Bacteria use sigma (σ) factors to recruit RNA polymerase (RNAP) to promoter regions of genes that need to be transcribed, with 60% bacteria containing at least one specialized σ factor, σ54, responsible for transcribing many stress response genes. The σ54-mediated transcription initiation requires specific AAA+ proteins (ATPases Associated with diverse cellular Activities) known as bacterial enhancer-binding proteins (bEBPs). DNA looping enables bEBP hexamers to engage and actively remodel the RNAP-σ54-DNA closed complex to convert it into an open complex. In this work we capture intermediate states of bEBPs in facilitating DNA opening and partial unfolding of σ54, and therefore link the ATPase activity to DNA opening and σ54 remodeling, which eventually lead to transcription activation.

To understand the structural basis and how DNA is stabilized in these complexes, we determined the structures of PspF1-275-RNAP-σ54-DNA containing mismatches between −11 and −8 [RPi(−11/−8)] and between −10 and −1 [RPi(−10/−1)]. In the RPi(−10/−1) complex, we also observe a range of PspF1-275 hexamer ring conformations with one resolved to higher resolution. Interestingly, in this conformation, the hexamer ring has similar tilt as that of RPi (−11/−8) at ~50° while the DNA is bent even further (>70°) compared to that RPi(−11/−8). Despite the conformational differences, similarly to RPi(−12/−11) structure, the protomer that engages with DNA is also at the highest position within the hexamer ring. In these complexes, we observe a previously unreported interaction between PspF and σ54 RpoN domain. This interaction is only possible with the tilted ring conformation, suggesting this interaction contributes to the stabilization of this ring conformation in both RPi(−11/−8) and RPi(−10/−1), giving rise to the higher-resolution reconstruction of these conformations. Given the PspF1-275 rings are in similar positions between RPi(−11/−8) and RPi(−10/−1) complexes, we could compare the relative positions of each protomer between RPi(−11/−8) and RPi(−10/−1). Compared to RPi(−11/−8), the position of the power stroke protomer (protomer 1) has shifted within the ring, with the protomer in position 2 now becoming the power stroke protomer (protomer 1 position) in, suggesting that these two complexes could represent two states as described in Fig. 3 after the hydrolysis of protomer 1. Interestingly, protomer 1 in RPi(−10/−1) is shifted significantly toward protomer 6 compared to that of RPi(−11/−8), with the distance between L1 of these two protomers reduced from 27 Å to 4 Å, consistent with our proposed mechanistic model that hydrolysis of protomer 1 at the top of the spiral causes it to relocate downward in the hexamer spiral. Significantly, we observe the σ54 N terminus is further shifted along the PspF hexamer in RPi(−11/−8) and RPi(−10/−1) compared to that of RPi(−12/−11).

>[6x]MAEYKDNLLGEANSFLEVLEQVSHLAPLDKPVLIIGERGTGKELIASRLHYLSSRWQGPFISLNCAALNENLLDSELFGHEAGAFTGAQKRHPGRFERADGGTLFLDELATAPMMVQEKLLRVIEYGELERVGGSQPLQVNVRLVCATNADLPAMVNEGTFRADLLDRLAFDVVQLPPLRERESDIMLMAEYFAIQMCREIKLPLFPGFTERARETLLNYRWPGNIRELKNVVERSVYRHGTSDYPLDDIIIDPFKRRPPEDAIAVSETTSLPTL;>MQGSVTEFLKPRLVDIEQVSSTHAKVTLEPLERGFGHTLGNALRRILLSSMPGCAVTEVEIDGVLHEYSTKEGVQEDILEILLNLKGLAVRVQGKDEVILTLNKSGIGPVTAADITHDGDVEIVKPQHVICHLTDENASISMRIKVQRGRGYVPASTRIHSEEDERPIGRLLVDACYSPVERIAYNVEAARVEQRTDLDKLVIEMETNGTIDPEEAIRRAATILAEQLEAFVDLRDVRQPEVKEEKPEFDPILLRPVDDLELTVRSANCLKAEAIHYIGDLVQRTEVELLKTPNLGKKSLTEIKDVLASRGLSLGMRLENWPPASIADE[2x];> MVYSYTEKKRIRKDFGKRPQVLDVPYLLSIQLDSFQKFIEQDPEGQYGLEAAFRSVFPIQSYSGNSELQYVSYRLGEPVFDVQECQIRGVTYSAPLRVKLRLVIYEREAPEGTVKDIKEQEVYMGEIPLMTDNGTFVINGTERVIVSQLHRSPGVFFDSDKGKTHSSGKVLYNARIIPYRGSWLDFEFDPKDNLFVRIDRRRKLPATIILRALNYTTEQILDLFFEKVIFEIRDNKLQMELVPERLRGETASFDIEANGKVYVEKGRRITARHIRQLEKDDVKLIEVPVEYIAGKVVAKDYIDESTGELICAANMELSLDLLAKLSQSGHKRIETLFTNDLDHGPYISETLRVDPTNDRLSALVEIYRMMRPGEPPTREAAESLFENLFFSEDRYDLSAVGRMKFNRSLLREEIEGSGILSKDDIIDVMKKLIDIRNGKGEVDDIDHLGNRRIRSVGEMAENQFRVGLVRVERAVKERLSLGDLDTLMPQDMINAKPISAAVKEFFGSSQLSQFMDQNNPLSEITHKRRISALGPGGLTRERAGFEVRDVHPTHYGRVCPIETPEGPNIGLINSLSVYAQTNEYGFLETPYRKVTDGVVTDEIHYLSAIEEGNYVIAQANSNLDEEGHFVEDLVTCRSKGESSLFSRDQVDYMDVSTQQVVSVGASLIPFLEHDDANRALMGANMQRQAVPTLRADKPLVGTGMERAVAVDSGVTAVAKRGGVVQYVDASRIVIKVNEDEMYPGEAGIDIYNLTKYTRSNQNTCINQMPCVSLGEPVERGDVLADGPSTDLGELALGQNMRVAFMPWNGYNFEDSILVSERVVQEDRFTTIHIQELACVSRDTKLGPEEITADIPNVGEAALSKLDESGIVYIGAEVTGGDILVGKVTPKGETQLTPEEKLLRAIFGEKASDVKDSSLRVPNGVSGTVIDVQVFTRDGVEKDKRALEIEEMQLKQAKKDLSEELQILEAGLFSRIRAVLVAGGVEAEKLDKLPRDRWLELGLTDEEKQNQLEQLAEQYDELKHEFEKKLEAKRRKITQGDDLAPGVLKIVKVYLAVKRRIQPGDKMAGRHGNKGVISKINPIEDMPYDENGTPVDIVLNPLGVPSRMNIGQILETHLGMAAKGIGDKINAMLKQQQEVAKLREFIQRAYDLGADVRQKVDLSTFSDEEVMRLAENLRKGMPIATPVFDGAKEAEIKELLKLGDLPTSGQIRLYDGRTGEQFERPVTVGYMYMLKLNHLVDDKMHARSTGSYSLVTQQPLGGKAQFGGQRFGEMEVWALEAYGAAYTLQEMLTVKSDDVNGRTKMYKNIVDGNHQMEPGMPESFNVLLKEIRSLGINIELEDE;> MKDLLKFLKAQTKTEEFDAIKIALASPDMIRSWSFGEVKKPETINYRTFKPERDGLFCARIFGPVKDYECLCGKYKRLKHRGVICEKCGVEVTQTKVRRERMGHIELASPTAHIWFLKSLPSRIGLLLDMPLRDIERVLYFESYVVIEGGMTNLERQQILTEEQYLDALEEFGDEFDAKMGAEAIQALLKSMDLEQECEQLREELNETNSETKRKKLTKRIKLLEAFVQSGNKPEWMILTVLPVLPPDLRPLVPLDGGRFATSDLNDLYRRVINRNNRLKRLLDLAAPDIIVRNEKRMLQEAVDALLDNGRRGRAITGSNKRPLKSLADMIKGKQGRFRQNLLGKRVDYSGRSVITVGPYLRLHQCGLPKKMALELFKPFIYGKLELRGLATTIKAAKKMVEREEAVVWDILDEVIREHPVLLNRAPTLHRLGIQAFEPVLIEGKAIQLHPLVCAAYNADFDGDQMAVHVPLTLEAQLEARALMMSTNNILSPANGEPIIVPSQDVVLGLYYMTRDCVNAKGEGMVLTGPKEAERLYRSGLASLHARVKVRITEYEKDANGELVAKTSLKDTTVGRAILWMIVPKGLPYSIVNQALGKKAISKMLNTCYRILGLKPTVIFADQIMYTGFAYAARSGASVGIDDMVIPEKKHEIISEAEAEVAEIQEQFQSGLVTAGERYNKVIDIWAAANDRVSKAMMDNLQTETVINRDGQEEKQVSFNSIYMMADSGARGSAAQIRQLAGMRGLMAKPDGSIIETPITANFREGLNVLQYFISTHGARKGLADTALKTANSGYLTRRLVDVAQDLVVTEDDCGTHEGIMMTPVIEGGDVKEPLRDRVLGRVTAEDVLKPGTADILVPRNTLLHEQWCDLLEENSVDAVKVRSVVSCDTDFGVCAHCYGRDLARGHIINKGEAIGVIAAQSIGEPGTQLTMRTFHIGGAASRAAAESSIQVKNKGSIKLSNVKSVVNSSGKLVITSRNTELKLIDEFGRTKESYKVPYGAVLAKGDGEQVAGGETVANWDPHTMPVITEVSGFVRFTDMIDGQTITRQTDELTGLSSLVVLDSAERTAGGKDLRPALKIVDAQGNDVLIPGTDMPAQYFLPGKAIVQLEDGVQISSGDTLARIPQESGGTKDITGGLPRVADLFEARRPKEPAILAEISGIVSFGKETKGKRRLVITPVDGSDPYEEMIPKWRQLNVFEGERVERGDVISDGPEAPHDILRLRGVHAVTRYIVNEVQDVYRLQGVKINDKHIEVIVRQMLRKATIVNAGSSDFLEGEQVEYSRVKIANRELEANGKVGATYSRDLLGITKASLATESFISAASFQETTRVLTEAAVAGKRDELRGLKENVIVGRLIPAGTGYAYHQDRMRRRAAG;> MARVTVQDAVEKIGNRFDLVLVAARRARQMQVGGKDPLVPEENDKTTVIALREIEEGLINNQILDVRERQEQQEQEAAELQAVTAIAEGRR;> MKQGLQLRLSQQLAMTPQLQQAIRLLQLSTLELQQELQQALESNPLLEQTDLHDEVEAKEVEDRESLDTVDALEQKEMPDELPLDASWDEIYTAGTPSGNGVDYQDDELPVYQGETTQTLQDYLMWQVELTPFTDTDRAIATSIVDAVDDTGYLTIQIEDIVDSIGDDEIGLEEVEAVLKRIQRFDPVGVAAKDLRDCLLIQLSQFAKETPWLEEARLIISDHLDLLANHDFRTLMRVTRLKEEVLKEAVNLIQSLDPRPGQSIQTSEPEYVIPDVLVRKVSGRWTVELNADSIPRLKINQQYAAMGNSARNDADGQFIRSNLQEARWLIKSLESRNDTLLRVSRCIVEQQQAFFEQGEEYMKPMVLADIAQAVEMHESTISRVTTQKYLHSPRGIFELKYFFSSHVNTEGGGEASSTAIRALVKKLIAAENPAKPLSDSKLTSMLSEQGIMVARRTVAKYRESLSIPPSNQRKQLV>MVAENQPGHIDQIKQTNAGAVYRLIDQLGPVSRIDLSRLAQLAPASITKIVREMLEAHLVQELEIKEAGNRGRPAVGLVVETEAWHYLSLRISRGEIFLALRDLSSKLVVEESQELALKDDSPLLDRIISHIDQFFIRHQKKLERLTSIAITLPGIIDTENGIVHRMPFYEDVKEMPLGEALEQHTGVPVYIQHDISAWTMAEALFGASRGARDVIQVVIDHNVGAGVITDGHLLHAGSSSLVEIGHTQVDPYGKRCYCGNHGCLETIASVDSILELAQLRLNQSMSSMLHGQPLTVDSLCQAALRGDLLAKDIITGVGAHVGRILAIMVNLFNPQKILIGSPLSKAADILFPVISDSIRQQALPAYSQHISVESTQFSNQGTMAGAALVKDAMYNGS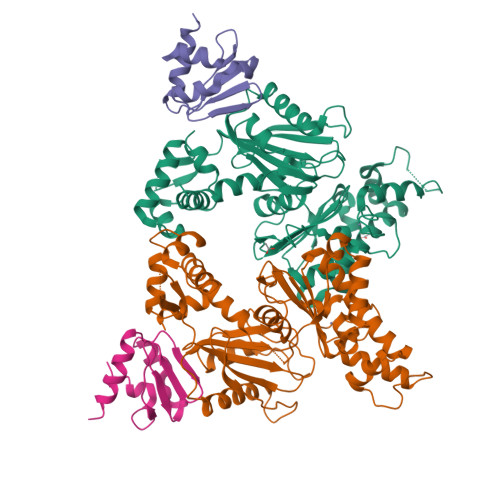LLIRLLQG[2x];>MAPALVAAFGGKENITNLDACITRLRVSVADVSKVDQAGLKKLGAAGVVVAGSGVQAIFGTKSDNLKTEMDEYIR[2x]> MDVVRASRNAKVKGKFRESYLSPAQSVKPKINTEEKLPREKLNPPTPSIYLESKRDAFSPVLLQFCTDPRNPITVIRGLAGSLRLNLGLFSTKTLVEASGEHTVEVRTQVQQPSDENWDLTGTRQIWPCESSRSHTTIAKYAQYQASSFQES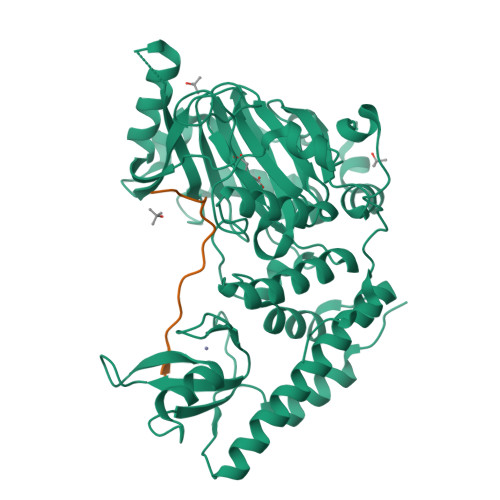LQEEKESEDEESEEPDSTTGTPPSSAPDPKNHHIIKFGTNIDLSDAKRWKPQLQELLKLPAFMRVTSTGNMLSHVGHTILGMNTVQLYMKVPGSRTPGHQENNNFCSVNINIGPGDCEWFAVHEHYWETISAFCDRHGVDYLTGSWWPILDDLYASNIPVYRFVQRPGDLVWINAGTVHWVQATGWCNNIAWNVGPLTAYQYQLALERYEWNEVKNVKSIVPMIHVSWNVARTVKISDPDLFKMIKFCLLQSMKHCQVQRESLVRAGKKIAYQGRVKDEPAYYCNECDVEVFNILFVTSENGSRNTYLVHCEGCARRRSAGLQGVVVLEQYRTEELAQAYDAFTLAPASTSRHHHHHH;> RIQLMTKAARKSAPATG> MALKDLFERDVQELEREGILFTTLEKLVAWGRSNSLWPATFGLACCAIEMMASTDARNDLARFGSEVFRASPRQADVMIV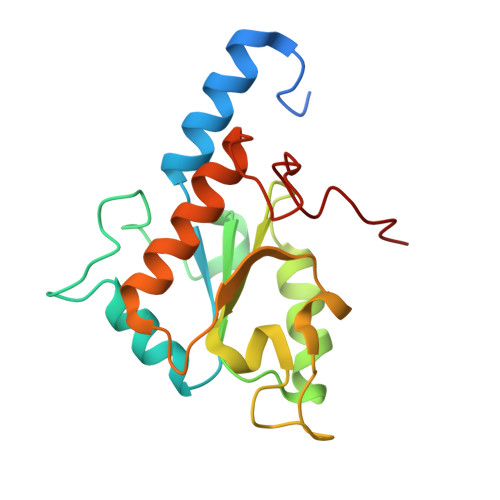AGRLSKKMAPVMRRVWEQMPDPKWVISMGACASSGGMFNNYAIVQNVDSVVPVDVYVPGCPPRPEALIYAVMQLQKKVRGQAYNERGERLPPVAAWKRTRG>MVSAVLRTILVTGGAGYIGSHTVLQLLQQGFRVVVVDNLDNASEAALARVAELAGHDGANLVFHKVDLRDRHALVDIFSSHRFEAVIHFAGLKAVGESVHKPLLYYDNNLVGTITLLEVMAANGCKKLVFSSSATVYGWPKEVPCTEEFPLCATNPYGRTKLVIEDICRDVHRSDPDWKIILLRYFNPVGAHPSGYIGEDPCGVPNNLMPYVQQVAVGRLPHLTVYGTDYSTKDGTGVRDYIHVVDLADGHIAALRKLYEDSDKIGCEVYNLGTGKGTSVLEMVAAFEKASGKKIPLVFAGRRPGDAEIVYAATAKAEKELKWKAKYGIEEMCRDLWNWASKNPYGYAGSRDNSK[2x]

BZU3 encodes a UDP-Glc 4-epimerase and plays a key role in controlling cell wall synthesis during the morphogenesis of maize stomata. It also catalyzes epimerization of UDP-N-acetylgalactosamine (UDP-GalNAc) to UDP-N-acetylglucosamine (UDP-GlcNAc), regulating N-glycosylation patterns of many proteins that may be involved in cell wall synthesis and signaling pathways. BZU3 formed a homo-dimer, with each protomer folded into two distinct structural units, the N-terminal NAD+ binding domain (residues 1-189) and the C-terminal sugar-binding domain (residues 190-355). The catalytic site was located in the cleft between these two structural domains.

To further address the molecular functions of BZU3, we solved the 3-D structures of the BZU3 protein, both in apo form and in complexes with NAD+/UDP-Glc and NAD+/UDP-GlcNAc, at resolutions of 2.6 Å, 1.25 Å, and 2.15 Å respectively. The homo-dimerization structure was consistent with in vivo bimolecular fluorescence complementation (BiFC) results. BZU3bzu3-2 failed to form homo-dimers, probably due to the frameshift which would be expected to alter the structural folding of its C-terminal domain. The maize BZU3 shared similar structures with the GALE proteins from humans and E. coli. The highly conserved NAD+ binding motifs (G13XXG16XXG19 and Y157XXXK161) of the UGE family were indicated in the aligned sequences.>SKKHTGYVGLKNQGATCYMNSLLQTLFFTNQLRKAVYMMPTEGDDSSKSVPLALQRVFYELQHSDKPVGTKKLTKSFGWETLDSFMQHDVQELCRVLLDNVENKMKGTCVEGTIPKLFRGKMVSYIQCKEVDYRSDRREDYYDIQLSIKGKKNIFESFVDYVAVEQLDGDNKYDAGEHGLQEAEKGVKFLTLPPVLHLQLMRFMYDPQTDQNIKINDRFEFPEQLPLDEFLQKTDPKDPANYILHAVLVHSGDNHGGHYVVYLNPKGDGKWCKFDDDVVSRCTKEEAIEHNYGG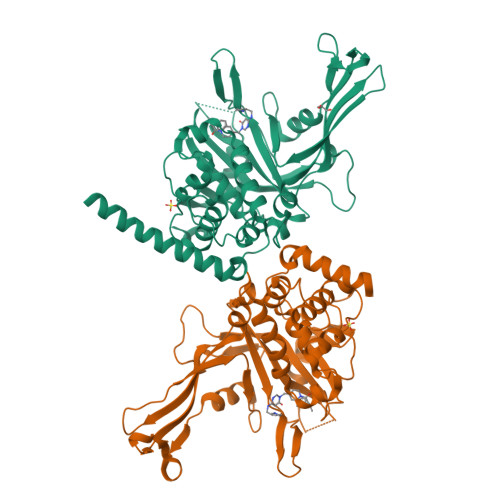HDDDLSVRHCTNAYMLVYIRESKLSEVLQAVTDHDIPQQLVERLQEEKRIEAQKRKERQEHHH[2x]> SDTRKKRKDPDSDDWSESNSKENKIDNKHLNLLSSDSEIEQDYQKAKKRKTSDL;> AELPQMTQQLNSDDMQEQLSATVKFRQILSREHRPPIDVVIQAGVVPRLVEFMRENQPEMLQLEAAWALTNIASGTSAQTKVVVDADAVPLFIQLLYTGSVEVKEQAIWALGNVAGDSTDYRDYVLQCNAMEPILGLFNSNKPSLIRTATWTLSNLCRGKKPQPDWSVVS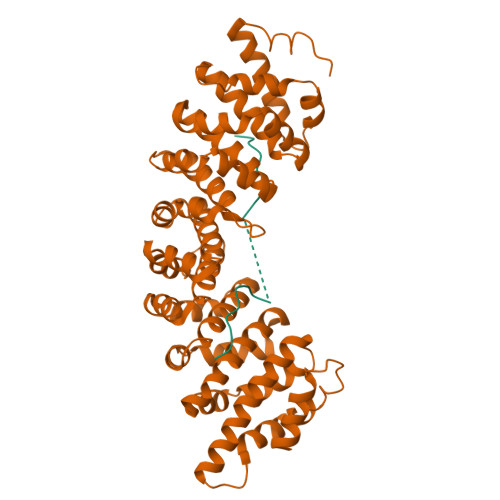QALPTLAKLIYSMDTETLVDACWAISYLSDGPQEAIQAVIDVRIPKRLVELLSHESTLVQTPALRAVGNIVTGNDLQTQVVINAGVLPALRLLLSSPKENIKKEACWTISNITAGNTEQIQAVIDANLIPPLVKLLEVAEYKTKKEACWAISNASSGGLQRPDIIRYLVSQGCIKPLCDLLEIADNRIIEVTLDALENILKMGEADKEARGLNINENADFIEKAGGMEKIFNCQQNENDKIYEKAYKIIETYF>[2x]SNVPHKSSLPEGIRPCTVLRIRGLVPPNASRFHVNLLCGEEQGSDAALHFNPRLDTSEVVFNSKEQG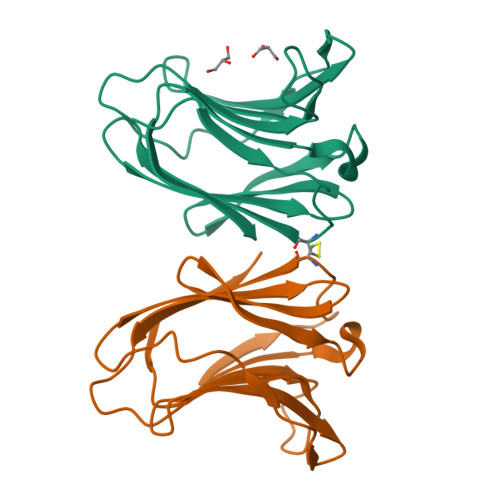SWGREERGPGVPFQRGQPFEVLIIASDDGFKAVVGDAQYHHFRHRLPLARVRLVEVGGDVQLDSVRIF>MNTNKATATYLKSIMLPETGPASIPDDITERHILKQETSSYNLEVSESGSGILVCFPGAPGSRIGAHYRWNANQTGLEFDQWLETSQDLKKAFNYGRLISRKYDIQSSTLPAGLYALNGTLNAATFEGSLSEVESLTYNSLMSLTTNPQDKVNNQLVTKGVTVLNLPTGFDKPYVRLEDETPQGLQSMNGAKMRCTAAIAPRRYEIDLPSQRLPPVPATGTLTTLYEGNADIVNSTTVTGDINFGLARQPADETTFHFQLDFMGLDNDVPVVTVVSSALATTDNHRGVSAKMTQSIPTENITKPITRVKLSYKINQQTAIDNV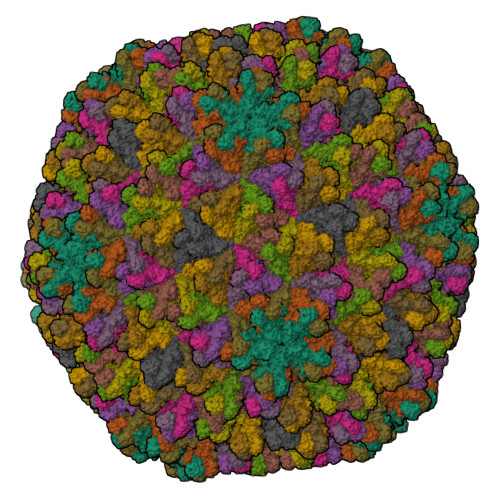ATLGTMGPASVSFSSGNGNVPGVLRPITLVAYEKMTPLSILTVAGVSNYELIPNPELLKNMVTRYGKYDPEGLNYAKMILSHREELDIRTVWRTEEYKERTRVFNEITDFSSDLPTSKAWGWRDIVRGIRKVAAPVLSTLFPMAAPLIGMADQFIGDLTKTNAAGGRYHSMAAGGRYKDVLESWA[13x]>[4x]MSNEIPKPVAPAPDILRCAYAELVVTDLAKSRNFYVDVLGLHVSYEDENQIYLRSFEEFIHHNLVLTKGPVAALKAMAFRVRTPEDVDKAEAYYQELGCRTERRKDGFVKGIGDALRVEDPLGFPYEFFFETTHVERLHMRYDLYSAGELVRLDHFNQVTPDVPRGRKYLEDLGFRVTEDIQDDEGTTYAAWMHRKGTVHDTALTGGNGPRLHHVA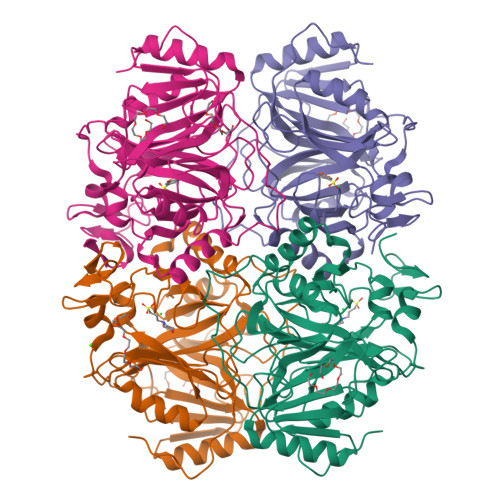FSTHEKHNIIQICDKMGALRISDRIERGPGRHGVSNAFYLYILDPDNHRIEIYTQDYYTGDPDNPTITWNVHDNQRRDWWGNPVVPSWYTEASKVLDLDGNVQEIIERTDDSELEVTIGADGFSFTRAGDEDGSYHGQASKGFKLGNQL> MKLLQRGVALALLTTFTLASETALAYEQDKTYKITVLHTNDHHGHFWRNEYGEYGLAAQKTLVDGIRKEVAAEGGSVLLLSGGDINTGVPESDLQDAEPDFRGMNLVGYDAMAIGNHEFDNPLTVLRQQEKWAKFPLLSANIYQKSTGERLFKPWALFKRQDLKIAVIGLTTDDTAKIGNPEYFTDIEFRKPADEAKLVIQELQQTEKPDIIIAATHMGHYDNGEHGSNAPGDVEMARAL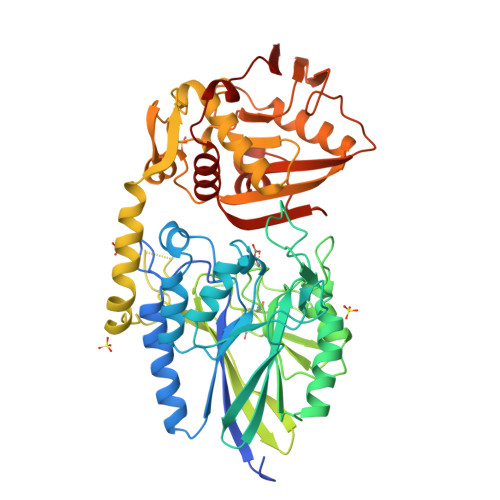PAGSLAMIVGGHSQDPVCMAAENKKQVDYVPGTPCKPDQQNGIWIVQAHEWGKYVGRADFEFRNGEMKMVNYQLIPVNLKKKVTWEDGKSERVLYTPEIAENQQMISLLSPFQNKGKAQLEVKIGETNGRLEGDRDKVRFVQTNMGRLILAAQMDRTGADFAVMSGGGIRDSIEAGDISYKNVLKVQPFGNVVVYADMTGKEVIDYLTAVAQMKPDSGAYPQFANVSFVAKDGKLNDLKIKGEPVDPAKTYRMATLNFNATGGDGYPRLDNKPGYVNTGFIDAEVLKAYIQKSSPLDVSVYEPKGEVSWQ N-[(S)-[(2S)-2-(benzoylamino)-2-carboxyethoxy](hydroxy)phosphoryl]-L-glutamic 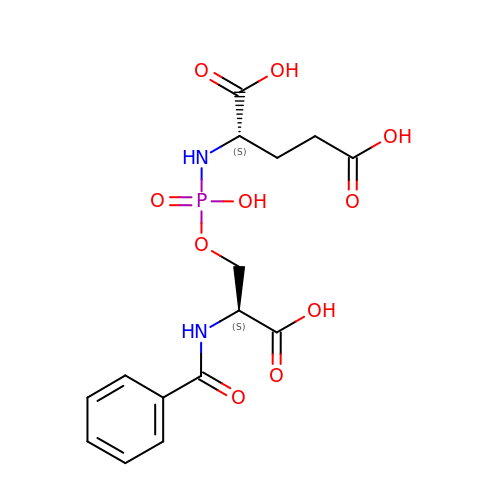acid | C15 H19 N2 O10 P | FMKMCQXFKJRGIQ-QWRGUYRKSA-N> MGHHHHHHHHH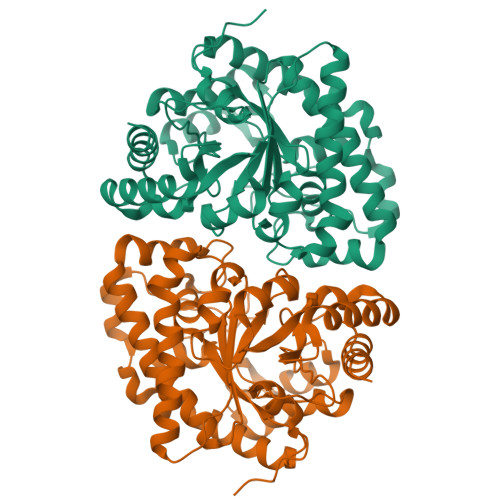HSSGHIEGRHMEANGLGPQGFPELKNDTFLRAAWGEETDYTPVWCMRQAGRYLPEFRETRAAQDFFSTCRSPEACCELTLQPLRRFPLDAAIIFSDILVVPQALGMEVTMVPGKGPSFPEPLREEQDLERLRDPEVVASELGYVFQAITLTRQRLAGRVPLIGFAGAPWTLMTYMVEGGGSSTMAQAKRWLYQRPQASHQLLRILTDALVPYLVGQVVAGAQALQLFESHAGHLGPQLFNKLALPYIRDVAKQVKARLREAGLAPVPMIIFAKDGHFALEELAQAGYEVVGLDWTVAPKKARECVGKTVTLQGNLDPCALYASEEEIGQLVKQMLDDFGPHRYIANLGHGLYPDMDPEHVGAFVDAVHKHSRLLRQN The NIMA-related kinases (Neks) are a family of Ser/Thr protein kinases, first discovered in Aspergillus nidulans that are conserved in eukaryotes. Nek7 is 1 of 11 Neks found in humans, and contributes to the assembly of a robust mitotic spindle apparatus. Human Nek7 is a 34.5 kDa protein, comprising a singular canonical kinase domain made up of a small, 5 β-stranded, N-terminal lobe linked to a larger, mostly α-helical C-terminal lobe. The intervening cleft between the two lobes forms the ATP-binding pocket and active site in which phosphoryl transfer takes place.

We also determined the structure of Nek2 bound to the same inhibitor, to enable a direct comparison of binding modes. Compound 51 inhibits Nek2 with an IC50 of 1.42 µM, ∼50-fold more potently than Nek7SRS. The overall binding mode of compound 51 was similar in both structures: the purine scaffold lines up along the kinase hinge region; the substituted phenyl group sits on a Gly residue in the post-hinge region (G92 in Nek2, G117 in Nek7SRS), and the sulphonamide substituent points towards solvent; the cyclohexyl group fits between an Asp residue in the post-hinge region (D93 in Nek2, D118 in Nek7SRS) and the Gly-rich loop. As with previous structures of Nek2 bound to purine-based inhibitors, compound 51 forms three H-bonds with the hinge region of Nek2. The orientation of the substituted phenyl group of compound 51 is clearly different between the two structures: when bound to Nek2, the phenyl ring lies flat against Gly92, and the sulphonamide-amine substituent points towards Asp93; when bound to Nek7SRS or Nek7WT the phenyl ring is rotated so that the sulphonamide-amine points towards the N-lobe where it interacts with the side chain of Arg50. The equivalent residue to Leu113 of Nek7 in Nek2 is Tyr88, which partly fills the space occupied by the phenyl-sulfonamide of compound 51 in the Nek7-bound pose. A striking feature of the Nek2.51 structure is the contrast between the highly ordered core of the kinase and the poorly ordered C-helix. The C-helix in the Nek2-ADP structure has B-factors similar to the rest of the kinase core, whereas the C-helix in the Nek2.51 structure has the highest B-factors of any region modelled in the structure. There is no structural evidence that compound 51 destabilises the C-helix directly. Instead, it appears that it is unable to compensate for the loss of the stabilising effect of ADP on the C-helix.

> MPSRAEDYEVLYTIGTGSYGRCQKIRRKSDGKILVWKELDYGSMTEAEKQMLVSEVNLLRELKHPNIVRYYDRIIDRTNTTLYIVMEYCEGGDLASVITKGTKERQYLDEEFVLRVMTQLTLALKECHRRSDGGHTVLHRDLKPANVFLDGKQNVKLGDFGLARILNHDTSFAKTFVGTPYYMSPEQMNRMSYNEKSDIWSLGCLLYELCALMPPFTAFSQKELAGKIREGKFRRIPYRYSDELNEIITRMLNLKDYHRPSVEEILENPLILEHHHHHH>[2x]ILKPGEKLPQDKLEELKKINDAVKKTK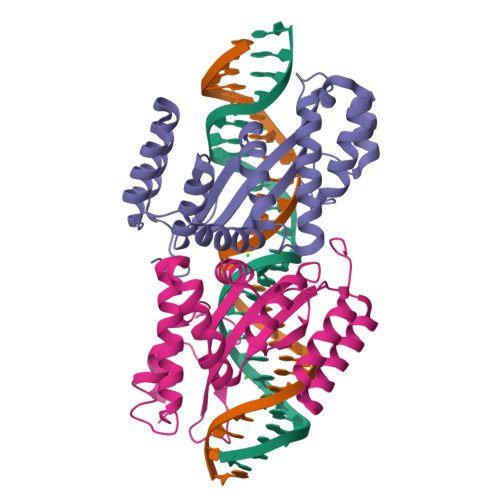NFSKYLIDLRKLFQIDEVQVTSESKLFLAGFLEGEASLNISTKKLATSKFGLVVDPEFNVTRHVNGVKVLYLALEVFKTGRIRHKSGSNATLVLTIDNRQSLEEKVIPFYEQYVVAFSSPEKVKRVANFKALLELFNNDAHQDLEQLVNKILPIWDQMRKQQGQSNEGFPNLEAAQDFAR>[4x]HHHHHHGMASMTGGQQMGRDLYDDDDKSRLQSNRIMGFAEARVLDAGVFPNVTNINSDKLLGGLLASGFDEDSCLSRYQSVHYRKPSPYKPSSYLISKLRNYEKLHKRCGPGTESYKKALKQLDQEHIDGDGECKYVVWISFSGLGNRILSLASVFLYALLTDRVLLVDRGKDMDDLFCEPFLGMSWLLPLDFPMTDQFDGLNQESSRCYGYMVKNQVIDTEGTLSHLYLHLVHDYGDHDKMFFCEGDQTFIGKVPWLIVKTDNYFVPSLWLIPGFDDELNKLFPQKATVFHHLGRY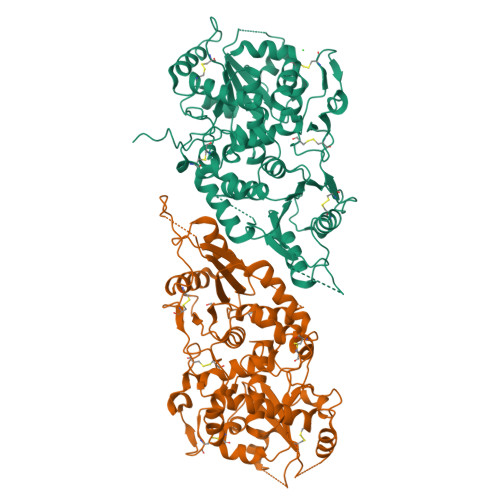LFHPTNQVWGLVTRYYEAYLSHADEKIGIQVRVFDEDPGPFQHVMDQISSCTQKEKLLPEVDTLVERSRHVNTPKHKAVLVTSLNAGYAENLKSMYWEYPTSTGEIIGVHQPSQEGYQQTEKKMHNGKALAEMYLLSLTDNLVTSAWSTFGYVAQGLGGLKPWILYRPENRTTPDPSCGRAMSMEPCFHSPPFYDCKAKTGIDTGTLVPHVRHCEDISWGLKLV Copper nitrite reductase (CuNiR) is part of the microbial respiratory N-oxide reduction denitrification pathway and catalyses the reduction of nitrite to form nitric oxide, a process with key agronomic and environmental impacts. CuNiRs are homotrimers, where each monomer contains a type 1 Cu centre (T1Cu) with a role in electron transfer and a catalytic type 2 copper centre (T2Cu) where nitrite binds and is converted to nitric oxide. The T2Cu centre has Cu(His)3–H2O ligation and nitrite binding displaces the H2O ligand. Rapid, shutterless X-ray detector technology on a synchrotron MX beamline was exploited to perform low-dose serial crystallography on a single copper nitrite reductase crystal, which survived long enough for 45 consecutive 100 K X-ray structures to be collected at 1.07–1.62 Å resolution, all sampled from the same crystal volume. This serial crystallography approach revealed the gradual conversion of the substrate bound at the catalytic type 2 Cu centre from nitrite to nitric oxide, following reduction of the type 1 Cu electron-transfer centre by X-ray-generated solvated electrons.

By ds4 (2.76 MGy accumulated dose) the nitrite had stabilized into a single ‘side-on’ conformation as observed previously in wild-type AcNiR structures. By ds4, the nitrite population converges into the ‘side-on’ NO2 conformation similar to that observed in previous studies, where it remains for a further six data sets. The conformation of Asp98 favours the proximal position at ∼0.6 occupancy between ds4 and ds10.

> DISTLPRVKVDLVKPPFVHAHDQVAKTGPRVVEFTMTIEEKKLVIDREGTEIHAMTFNGSVPGPLMVVHENDYVELRLINPDTNTLLHNIDFHAATGALGGGALTQVNPGEETTLRFKATKPGVFVYHCAPEGMVPWHVTSGMNGAIMVLPRDGLKDEKGQPLTYDKIYYVGEQDFYVPKDEAGNYKKYETPGEAYEDAVKAMRTLTPTHIVFNGAVGALTGDHALTAAVGERVLVVHSQANRDTRPHLIGGHGDYVWATGKFRNPPDLDQETWLIPGGTAGAAFYTFRQPGVYAYVNHNLIEAFELGAAGHFKVTGEWNDDLMTSVVKPAS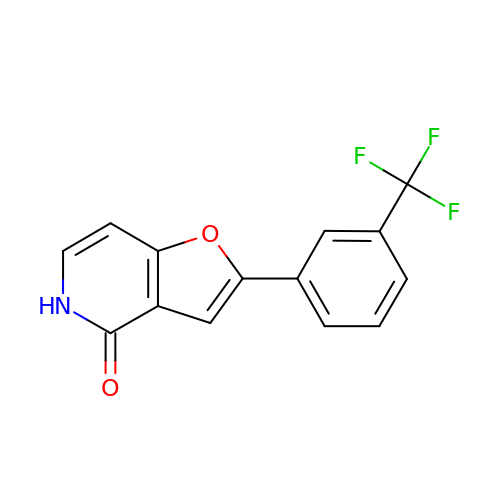2-[3-(trifluoromethyl)phenyl]furo[3,2-c]pyridin-4(5H)-one | C14 H8 F3 N O2 | ICVXPLDIRPNIOG-UHFFFAOYSA-N Adhesive chaperone-usher pili are long, supramolecular protein fibers displayed on the surface of many bacterial pathogens. The type 1 and P pili of uropathogenic Escherichia coli (UPEC) play important roles during urinary tract colonization, mediating attachment to the bladder and kidney, respectively. FimA (type 1 pilus) and PapA (P pilus) assemble into a ∼1,000-subunit long helically coiled quaternary structure of ∼3–4 subunits per turn known as the rod (Habenstein et al., 2015, Hospenthal et al., 2017, Hospenthal et al., 2016). The biomechanical properties of the helical pilus rods allow them to reversibly uncoil in response to flow-induced forces, allowing UPEC to retain a foothold in the unique and hostile environment of the urinary tract.

Here we present the 4.2-Å resolution cryoelectron microscopy (cryo-EM) structure of the related type 1 pilus rod. Type 1 pili were expressed and assembled on the Escherichia coli cell surface, from which they were sheared and purified by density gradient centrifugation as described in STAR Methods. The resulting electron density map was resolved to an overall resolution of 4.2 Å, which is consistent with the map showing clearly separated strands and visible density for bulky side chains. The pilus rod is ∼72 Å in diameter and contains a hollow central lumen, which is ∼14 Å wide. Overall, the type 1 pilus is a right-handed superhelical assembly comprising 3.13 subunits per turn with an axial rise of 8.0 Å per subunit and a pitch of 25 Å. An extensive subunit-subunit interaction network maintains the integrity of the superhelical quaternary structure, where each subunit interacts with a total of eight other subunits, four preceding and four succeeding subunits (n interacts with +1, +2, +3, +4 and −1, −2, −3, −4). By far the largest contribution to the subunit-subunit interaction network is made by the main stacking interface between every n and n+3 subunit pair. The majority of this interface is formed by residues on the loops linking β strands C and D (βC-βD loop) and D and E (βD-βE loop). By contrast, the N-terminal portion of the FimA Nte lies flat against the remainder of the FimA pilin fold. In turn, this implies that the stacking interface is stronger in type 1 pili (Andersson et al., 2008, Andersson et al., 2007). These findings are indeed supported by our cryo-EM structure of the type 1 pilus rod, which has a larger buried surface area (1,616.2 Å2) in the n and n+3 (stacking) interface than the P pilus (1,453.0 Å2) (Hospenthal et al., 2016).

>AATTVNGGTVHFKGEVVNAACAVDAGSVDQTVQLGQVRTASLAQEGATSSAVGFNIQLNDCDTNVASKAAVAFLGTAIDAGHTNVLALQSSAAGSATNVGVQILDRTGAALTLDGATFSSETTLNNGTNTIPFQARYFATGAATPGAANADATFKVQYQ[6x]> SHMGQGGSNPKFENIAEGLRALLARSHVERTTDEGTWVAGVFVYGGSKTSLYNL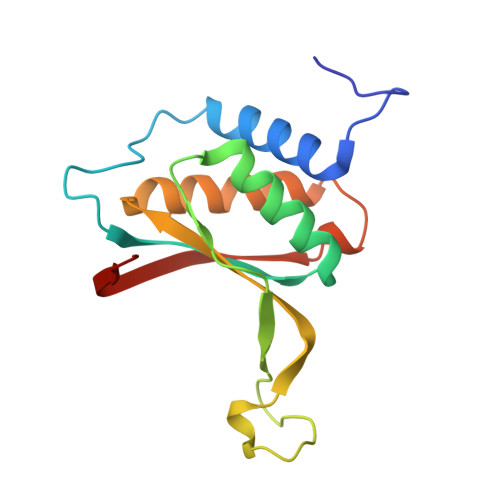RRGTALAIPQCRLTPLSRLPFGMAPGPGPQPGPLRESIVCYFMVFLQTHIFAEVLKDAIKDLVMTKPAPTCNIRVTVCSFDDGVDLP> SPQPLEQIKLSESQLSGRVGMIEMDLASGRTLTAWRADERFPMMSTFKVVLCGAVLARVDAGDEQLERKIHYRQQDLVKYSPVS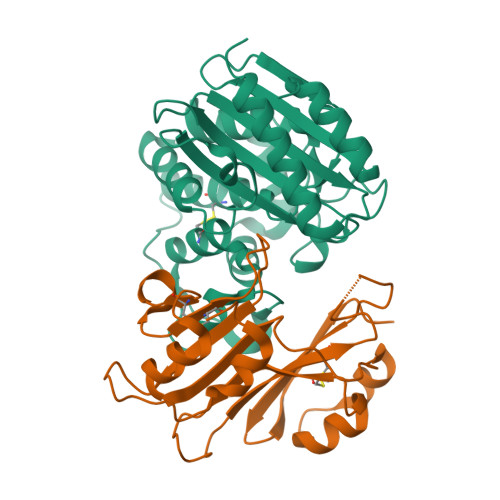EKHLADGMTVGELCAAAITMSDNSAANLLLATVGGPAGLTAFLRQIGDNVTRLDRWETELNEALPGDARDTTTPASMAATLRKLLTSQRLSARSQRQLLQWMVDDRVAGPLIRSVLPAGWFIADKTGAGERGARGIVALLGPNNKAERIVVIYLRDTPASMAERNQQIAGIGAALIEHWQR;> AGVMTGAKFTQIQFGMTRQQVLDIAGAENCETGGSFGDSIHCRGHAAGDYYAYATFGFTSAAADAKVDSKSQEKLLAPSAPTLTLAKFNQVTVGMTRAQVLATVGQGSCTTWSEYYPAYPSTAGVTLSLSCFDVDGYSSTGFYRGSAHLWFTDGVLQGKRQWDLV3-quinolin-6-yl-5-quinolin-7-yl-benzoic 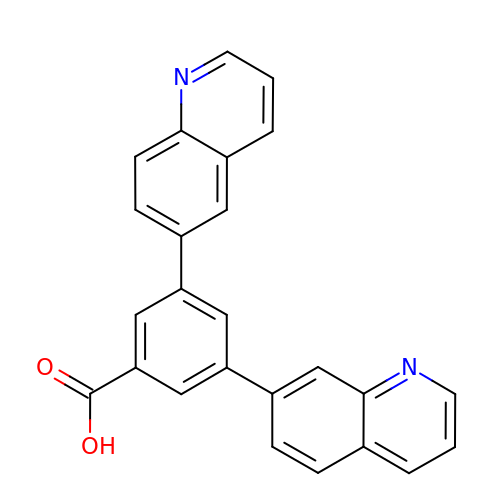acid | C25 H16 N2 O2 | OROXLWZECIFWHN-UHFFFAOYSA-N> ARIDPTKKGRRNRFKWGPASQQILFQA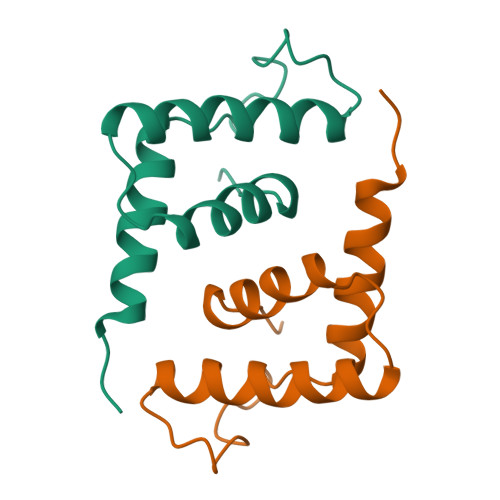YERQKNPSKEERETLVEECNRAECIQRGVSPSQAQGLGSNLVTEVRVYNWFANRRKEEAFRHKLAMDTYKLN> MGHHHHHHSGIALSRLAQERRAWRKDHPFGFVAVPTKNPDGTMNLMNWECAIPGKKGTPWEGGLFKLRMLFKDDYPSSPPKCKFEPPLFHPNVYPSGTVCLSILEEDKDWRPAITIKQILLGIQELLNEPNIQDPKQAEAYTIYCQNRVEYEKRVRAQAKKFAPS;> MGSSHHHHHHEGEYIKLKVIGQDSSEIHFKVKMTTHLKKLKESYCQRQGVPMNSLRFLFEGQRIADNHTPKELGMEEEDVIEVYQEQTGG

Protein SUMOylation is a ubiquitylation-like post-translational modification (PTM) that is synthesized through an enzymatic cascade involving an E1 (SAE1:SAE2), an E2 (UBC9), and various E3 enzymes. In the final step of this process, the small ubiquitin-like modifier (SUMO) is transferred from the UBC9∼SUMO thioester onto a lysine residue of a protein substrate. As the UBC9∼SUMO thioester is chemically unstable, a stable mimetic is desirable for structural studies of UBC9∼SUMO alone and in complex with a substrate and/or an E3 ligase. Here, we reproduce and further investigate this approach using the human SUMOylation system and characterize the resulting mimetic of human UBC9∼SUMO1.

The structure of the UBC9–SUMO1 molecule (i.e., auto-SUMOylated UBC9 K14R A129K) was solved at a 2.85-Å resolution in the P212121 spacegroup. The covalent link between lysine introduced in position 129 of UBC9 and G97 of SUMO1 is visible, too, but the C-terminal residues of SUMO1 exhibit high B-factors due to their flexibility. The Nζ atom of K129 is only 4 Å from the Sγ atom of C93, explaining why K129—which could move even closer when adopting a different rotamer—efficiently accepts SUMO1 from C93. Comparing our structure to those of free WT human UBC9 that were previously solved in two different space groups shows that C93 is shifted by about 1 Å compared to its position in free WT UBC9. This means that, in our conjugate, SUMO1 is linked 3 Å away from its attachment site in a real UBC9∼SUMO1 thioester conjugate, suggesting that our conjugate should serve as a suitable structural mimetic. C52 of SUMO1 and C138 of UBC9 (both from the same UBC9-SUMO1 molecule) are relatively close to each other in space, with a distance of ∼6 Å between their sulfur atoms. There is also unassigned electron density between the two cysteines, which we hypothesize could correspond to a DTT molecule that crosslinked these two cysteine residues in a portion of molecules in the crystal. Our mimetic does not adopt the closed conformation observed for activated E2∼modifier molecules, instead featuring an open conformation. This is consistent with the idea that, in the absence of an E3 ligase, the thioester (or, in this case, its mimetic) samples various conformations. When scrutinizing crystal contacts, we observed that UBC9–SUMO1 molecules form a chain: UBC9–SUMO1:UBC9–SUMO1:UBC9–SUMO1… (where “–“ denotes a covalent and “:” a noncovalent interaction). In this chain, SUMO1 from one covalent conjugate is noncovalently bound to UBC9 from a neighboring mimetic molecule through the well-characterized backside interaction.> MEVEPPLYPVAGAAGPQGDEDRHGVPDGPEAPLDELVGAYPNYNEEEEERRYYRRKRLGVVKNVLAASTGVTLTYGVYLGLLQMQLILHYDETYREVKYGNMGLPDIDSKMLMGINVTPIAALLYTPVLIRFFGTKWMMFLAVGIYALFVSTNYWERYYTLVPSAVALGMAIVPLWASMGNYITRMSQKYYEYSHYKEQDEQGPQQRPPRGSHAPYLLVFQAIFYSFFHLSFACAQLPMIYFLN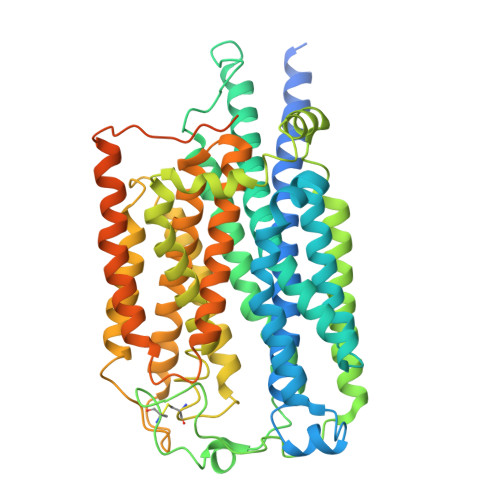NYLYDLNHTLINVQSCGTKSQGILNGFNKTVLRTLPRSKNLIVVESVLMAVAFLAMLMVLGLCGAAYRPTEEIDLRSVGWGNIFQLPFKHVRDFRLRHLVPFFIYSGFEVLFACTGFALGYGVCSMGLERLAYLLIAYSLGASASSVLGLLGLWLPRSVPLVAGAGLHLLLTLSLFFWAPAPRVLQHSWIFYFVAALWGVGSALNKTGLSTLLGILYEDKERQDFIFTIYHWWQAVAIFVVYLGSSLPMKAKLAVLLVTLVAAAASYLWMEQKLQQGLVPRQPRIPKPQHKVRGYRYLEEDNSDESDMEGEQGQGDCAEDEAPQAGPLGAEPAGPCRKPCPYEQALGGDGPEEQ> MGPLLVWHRGDLRLHDHPALLEALARGPVVGLVVLDPNNLKTTPRRRAWFLENVRALREAYRARGGALWVLEGLPWEKVPEAARRLKAKAVYALTSHTPYGRYRDGRVREALPVPLHLLPAPHLLPPDLPRAYRVYTPFSRLYRGAAPPLPPPEALPKGPEEGEIPREDPGLPLPEPGEEAALAGLRAFLEAKLPRYAEERDRLDGEGGSRLSPYFALGVLSPRLAAWEAERRGGEGARKWVAELLWRDFSYHLLYHFPWMAERPLDPRFQAFPWQEDEALFQAWYE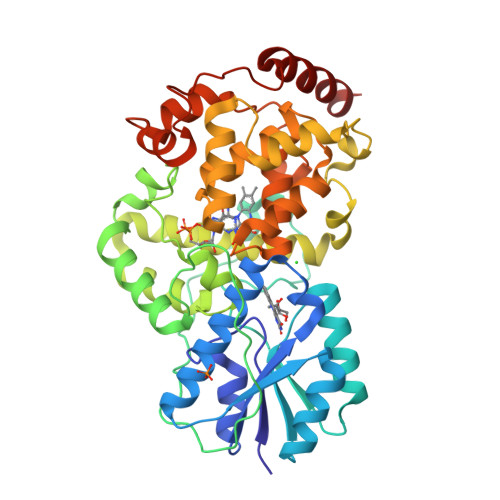GKTGVPLVDAAMRELHATGFLSNRARMNAAQFAVKHLLLPWKRCEEAFRHLLLDGDRAVNLQGWQWAGGLGVDAAPYFRVFNPVLQGERHDPEGRWLKRWAPEYPSYAPKDPVVDLEEARRRYLRLARDLARG>MSLSESLAKYGITGATNIVHNPSHEELFAAETQASLEGFEKGTVTEMGAVNVMTGVYTGRSPKDKFIVKNEASKEIWWTSDEFKNDNKPVTEEAWAQLKALAGKELSNKPLYVVDLFCGANENTRLKIRFVMEVAWQAHFVTNMFIRPTEEELKGFEPDFVVLNASKAKVENFKELGLNSETAVVFNLAEKMQIILNTWYGGEMKKGMFSMMNFYLPLQGIAAMHCSANTDLEGKNTAIFFGLSGTGKTTLSTDPKRLLIGDDEHGWDDDGVFNFEGGCYAKVINLSKENEPDIWGAIKRNALLENVTVDANGKVDFADKSVTENTRVSYPIFHIKNIVKPVSKAPAAKRVIFLSADAFGVLPPVSILSKEQTKYYFLSGFTAKLAGTERGITEPTPTF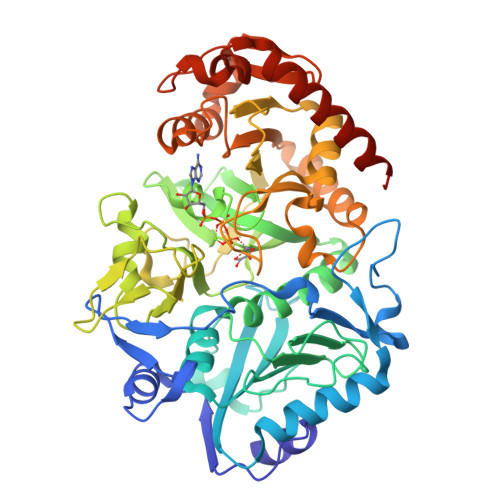SSCFGAAFLTLPPTKYAEVLVKRMEASGAKAYLVNTGWNGTGKRISIKDTRGIIDAILDGSIDTANTATIPYFNFTVPTELKGVDTKILDPRNTYADASEWEVKAKDLAERFQKNFKKFESLGGDLVKAGPQL[2x]>[12x]GSHMPKRTFTKEDIRKFAEEENVRYLRLQFTDIL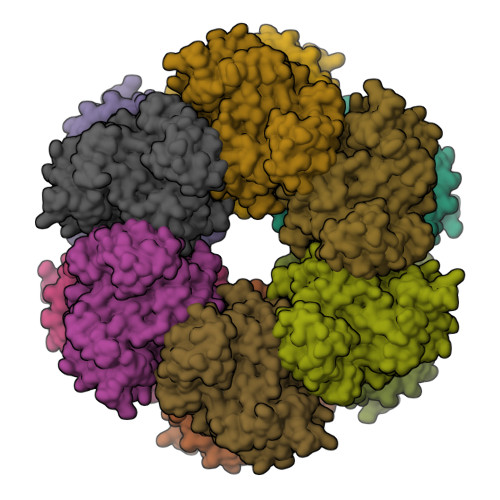GTIKNVEVPVSQLEKVLDNEMMFDGSSIEGFVRIEESDMYLHPDLDTWVIFPWTAGQGKVARLICDVYKTDGTPFEGDPRANLKRVLKEMEDLGFTDFNLGPEPEFFLFKLDEKGEPTLELNDDGGYFDLAPTDLGENCRRDIVLELEDMGFDIEASHHEVAPGQHEIDFKYADAVTACDNIQTFKLVVKTIARKHNLHATFMPKPLFGVNGSGMHFNVSLFKGKENAFFDPNTEMGLTETAYQFTAGVLKNARGFTAVCNPLVNSYKRLVPGYEAPCYIAWSGKNRSPLIRVPSSRGLSTRIEVRSVDPAANPYMALAAILEAGLDGIKNKLKVPEPVNQNIYEMNREEREAVGIQDLPSTLYTALKAMRENEVIKKALGNHIYNQFINSKSIEWDYYRTQVSEWERDQYMKQY>SMSLPKVMIVVGGQAPKAIRSVECYDFEEDRWDQIAELPSRRCRAGVVFMAGHVYAVGGFNGSLRVRTVDVYDGVKDQWTSIASMQERRSTLGAAVLNDLLYAVGGFDGSTGLASVEAYSYKTNEWFFVAPMNTRRSSVGVGVVEGKLYAVGGYDGASRQCLSTVEQYNPATNEWIYVADMSTRRSGAGVGVLSGQLYATGGHDGPLVRKSVEVYDPGTNTWKQVADMNMCRRNAGVCAVNGLLYVVGGDDGSCNLASVEYYNPVTDKWTLLPTNMSTGRSYAGVAVIHKSL[2x];>[2x]EPEEPEADQHQ

KLHL3 is the substrate-recognition subunit of the ubiquitin ligase complex, recruiting substrates for ubiquitylation via its associated Kelch domain. KLHL2 shares 84% sequence identity with KLHL3 across the Kelch domain, and 86% identity overall. KLHL2 has also been implicated recently as a CUL3 substrate adaptor for WNK kinases. We determined the high-resolution crystal structures of the Kelch domains of human KLHL3 and KLHL2 in separate complexes with the 11-residue WNK4 degron motif.

The KLHL2 structure was solved at 1.6 Å (1 Å=0.1 nm) resolution in space group P43212, whereas the structure of KLHL3 was determined at 1.8 Å in space group P212121. Similarly, residues 296–299 and 586–587 of KLHL3 could not be modelled into the KLHL3–WNK4 complex, and WNK4 residues 566–567 and the side chains of Glu559 and Glu560 were also not defined. The KLHL2 and KLHL3 structures were determined at pH 7.5 and pH 4.3 respectively, which probably contributes to differences in the resolution of particular residues. For example, protonation of WNK4 His566 may explain why this residue is not clearly resolved in the crystal structure of the KLHL3 complex. The binding interface between KLHL3 and WNK4 spans all six Kelch repeats and has a total buried surface area of 510 Å2, with blades II, III and IV participating in the greatest number of contacts. Among the KLHL3 residues, Arg360 contributes the greatest contact area and forms hydrogen bond interactions with WNK4 Glu557, as well as with the main chain atoms of WNK4 Pro558 and Glu560. For example, WNK4 Glu562 has the greatest contact area of any interface residue and protrudes into the cleft between blades III and IV to hydrogen bond with KLHL3 Ser432 (right-hand panel). Mutations have been described at both sites in patients with Gordon's syndrome (E562K and S432N respectively) and would probably introduce steric clashes, as well the loss of hydrogen-bond formation. Perhaps the most notable interaction is the salt bridge formed between KLHL3 Arg528 and WNK4 Asp564. Finally, a buried water molecule is observed to mediate hydrogen bonding between WNK4 Ala563 and the side chains of KLHL3 Ser432 and Ser433 (right-hand panel).> MQTSARNQWFGTITARDHDDVQQHVDVLLADGKTRLKVAITAQSGARLGLDEGKEVLILLKAPWVGITQ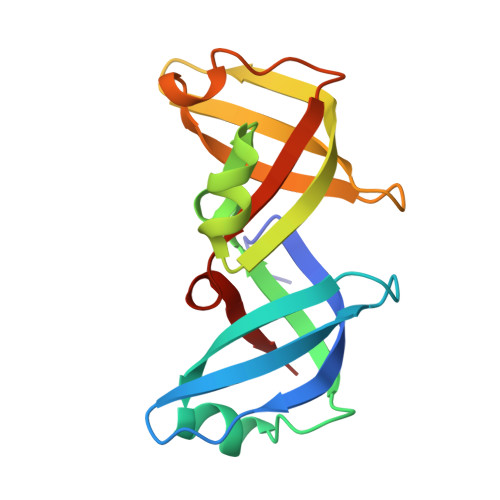DEAVAQNADNQLPGIISHIERGAEQCEVLMALPDGQTLCATVPVNEATSLEQGQNVTAYFNADSVIIATLC3,4,5-TRIMETHYL-1,3-THIAZOLE 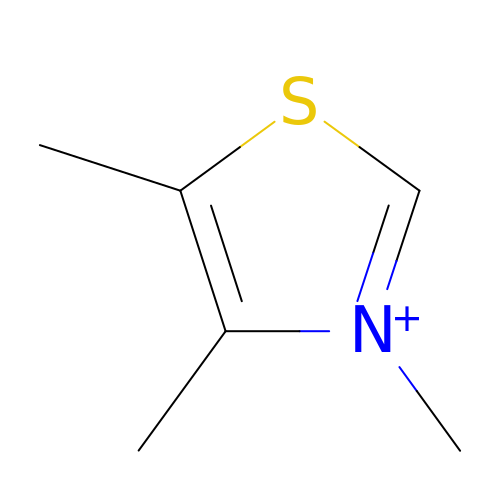| C6 H10 N S | LTPCOIDSGQEHKC-UHFFFAOYSA-N>[12x]KDSPIIEANGTLDELTSFIGEAKHYVDEEMKGILEEIQNDIYKIMGEIGSKGKIEGISEERIAWLLKLILRYMEMVNLKSFVLPGGTLESAKLDVCRTIARRALRKVLTVTREFGIGAEAAAYLLALSDLLFLLARVIEIE;>[12x]PHLVIEATANLRLETSPGELLEQANKALFASGQFGEADIKSRFVTLE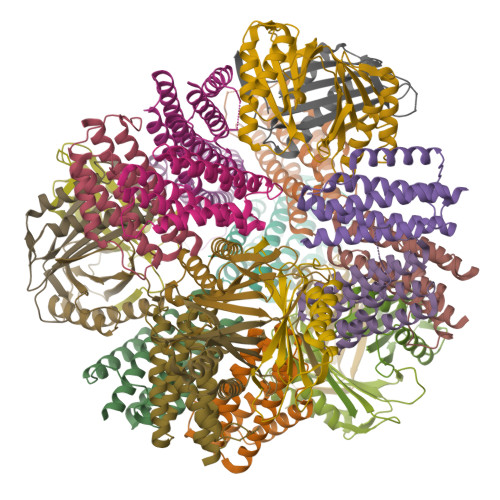AYRQGTAAVERAYLHACLSILDGRDIATRTLLGASLCAVLAEAVAGGGEEGVQVSVEVREMERLSYAKRVV> GLTIEAEPTELSYQDAL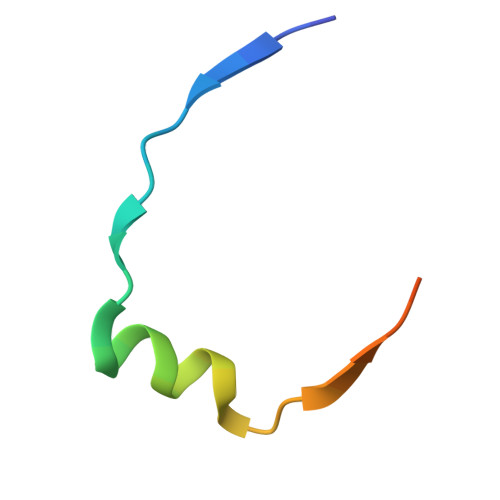EMLAESKPVSTTLSFER> MVERIEDLNLP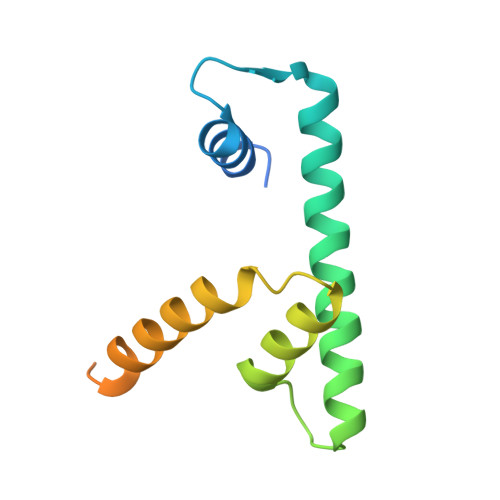NAVIGRLIKEALPESASVSKEARAAIARAASVFAIFVTSSSTALAHKQNHKTITAKDILQTLTELDFESFVPSLTQDLEVYRKVVKEKKESKASKKDSNTAENANASATATAEEAPE>SIPETQKGVIFYESHGKLEYKDIPVPKPKANELLINVKYSGVCHTDLHAWHGDWPLPVKLPLVGGHEGAGVVVGMGENVKGWKIGDYAGIKWLNGSCMACEYCELGNESNCPHADLSGYTHDGSFQQYATADAVQAAHIPQGTDLA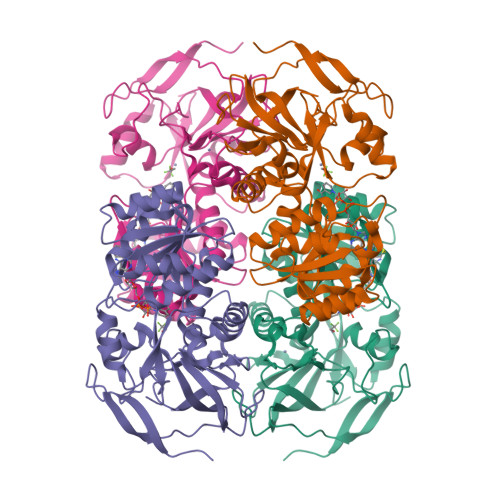QVAPILCAGITVYKALKSANLMAGHWVAISGAAGGLGSLAVQYAKAMGYRVLGIDGGEGKEELFRSIGGEVFIDFTKEKDIVGAVLKATDGGAHGVINVSVSEAAIEASTRYVRANGTTVLVGMPAGAKCCSDVFNQVVKSISIVGSYVGNRADTREALDFFARGLVKSPIKVVGLSTLPEIYEKMEKGQIVGRYVVDTSK[2x]>MGTFTQTNDPTIRKYVQSWQKLDVDEQLALFWFIYKEMGGAITPAAPGASTVSPAIAEGLFNQVKELNHEQQLQLQRDLIRRVDNQLSREYGSLGDTTKLLFWYLLSQGMDNATIVPFPADYKLSSES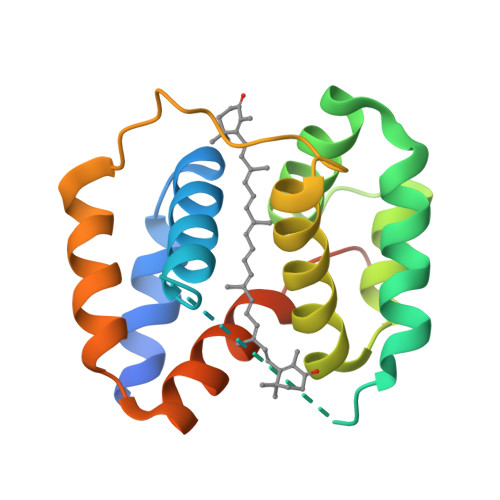QELLEGIKGLGFEQQITLFRDYVSPMGAEAKAGAEIHHHHHH[2x]> SNANEAQQYYLDADEAEAWIGEQELYVISDEIPKDEEGAIVMLKRHLRQQRAVEDYGRNIKQLASRAQGLLSAGHPEGEQIIRLQGQVDKHYAGLKDVACERKRKLENMYHLFQLKRETDDLEQWISEKELVASSPEMGQDFDHVTLLRDKFRDFARETGAIGQERVDNVNAFIERLIDAGHSEAATIAEWKDGLNEMWADLLELIDTRMQLLAASYDLHRYFYTGAEILGLIDEKHRELPEDVGLDASTAESFHRVHTAFER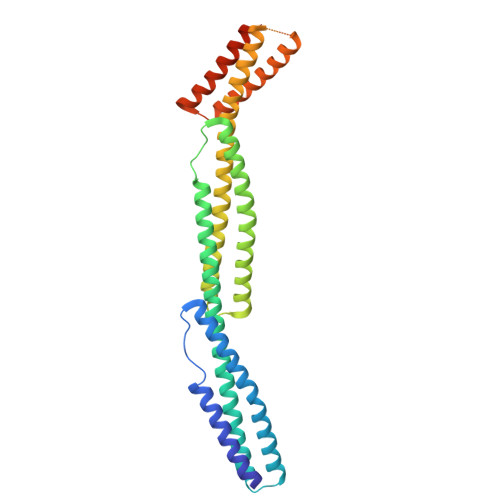DVHLLGVQVQQFQDVATRLQTAYAGEKAEAIQNKEQEVSAAWQALLDACAGRRTQLVDTADKF> MGDTFIRHIALLGFEKRFVPSQHYVYMFLVKWQDLSEKVVYRRFTEIYEFHKTLKEMFPIEAGAINPENRIIPHLPAPKWFDGQRAAENRQGTLTEYCSTLMSLPTKISRCPHLLDF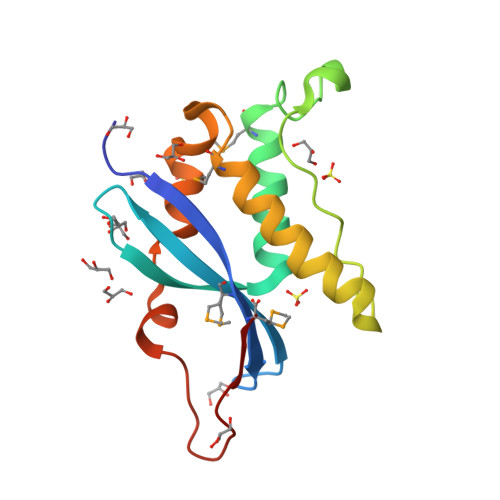FKVRPDDLKLPTDNQTKKPETYLM>ADNLAEFHVQNQECDSCHTPDGELSNDSLTYENTQCVSCHGTLAEVAETTKHEHYNAHASHFPGEVACTSCHSAHEKSMVYCDSCHSFDFNMPYAKKWLRDEPTIAELAKDKSERQAALASAPHDTVDVVVVGSGGAGFSAAISATDSGAKVILIEKEPVIGGNAKLAAGGMNAAWTDQQKAKKITDSPELMFEDTMKGGQNINDPALVKVLSSHSKDSVDWMTAMGADLTDVGMMGGASVNRAHRPTGGAGVGAHVVQVLYDNAVKRNIDLRMNTRGIEVLKDDKGTVKGILVKGMYKGYYWVKADAVILATGGFAKNNERVAKLDPSLKGFISTNQPGAVGDGLDVAENAGGALKDMQYIQAHPTLSVKGGVMV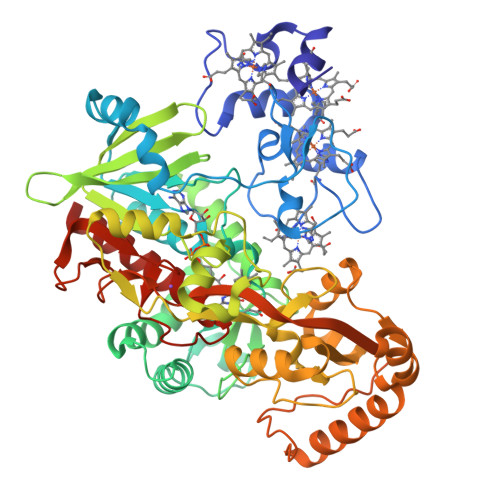TEAVRGNGAILVNREGKRFVNEITTKDKASAAILAQTGKSAYLIFDDSVRKSLSKIDKYIGLGVAPTADSLVKLGKMEGIDGKALTETVARYNSLVSSGKDTDFERPNLPRALNEGNYYAIEVTPGVHHTMGGVMIDTKAEVMNAKKQVIPGLYGAGEVTGGVHGANRLGGNAISDIITFGRLAGEEAAKYSKKN[2x]> SLYPKLFQKNLDPDVFNQIVKILHDFYIEKEKPLLIFEILQ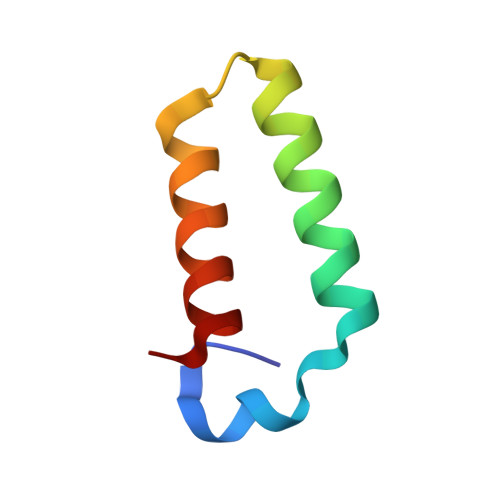RLSELKRFD7-{[(3-fluorophenyl)amino]methyl}quinolin-2-amine 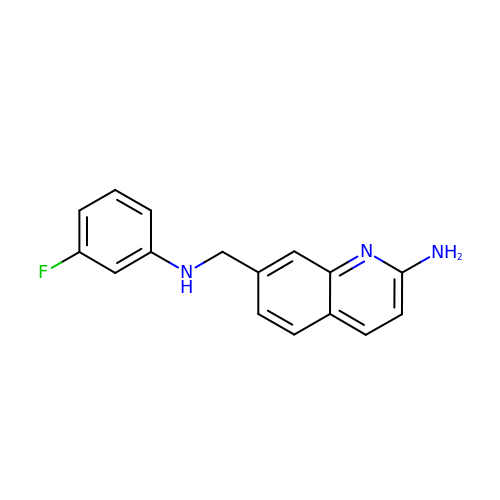| C16 H14 F N3 | UVVDQBVYPPCDJF-UHFFFAOYSA-N>[4x]GSAFFDEKEDTCAAVGEISVNTSVAFLPYMESVFEEVFKLLECPHLNVRKAAHEALGQFCCALHKACQSCPSEPNTAALQAALARVVPSYMQAVNRERERQVVMAVLEALTGVLRSCGTLTLKPPGRLAELCGVLKAVLQRKTACQDTDEEEEEEDDDQAEYDAMLLEHAGEAIPALAAAAGGDSFAPFFAGFLPLLVCKTKQGCTVAEK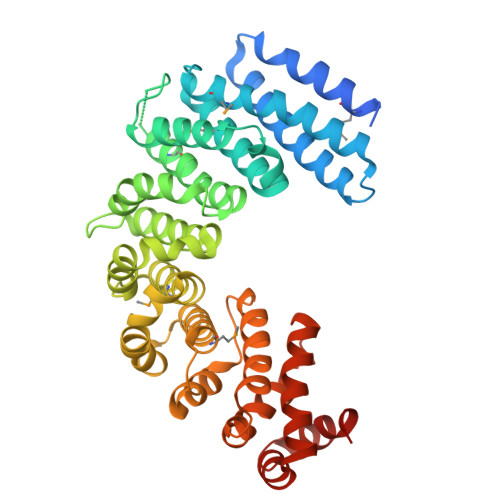SFAVGTLAETIQGLGAASAQFVSRLLPVLLSTAQEADPEVRSNAIFGMGVLAEHGGHPAQEHFPKLLGLLFPLLARERHDRVRDNICGALARLLMASPTRKPEPQVLAALLHALPLKEDLEEWVTIGRLFSFLYQSSPDQVIDVAPELLRICSLILADNKIPPDTKAALLLLLTFLAKQHTDSFQAALGSLPVDKAQELQAVLGLS> AEGTVSSSTDAL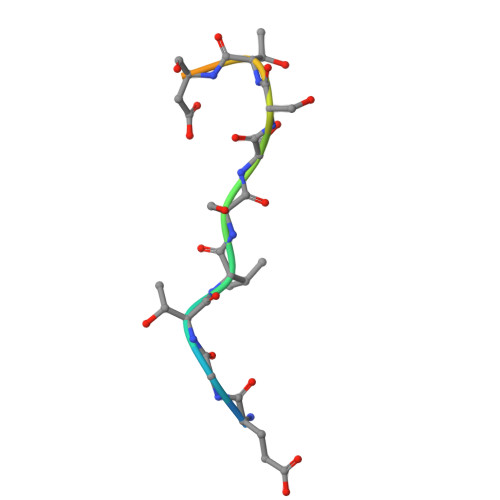PCI The ERK5 protein, which is encoded by the MAPK7 gene, comprises an N-terminal kinase domain and a large C-terminal domain containing transcriptional transactivating functionality and nuclear localization and export sequences (NLS/NES). ERK5 is the effector kinase of a canonical kinase module comprising MEK (MAPK/ERK kinase) 5, MEKK (MEK kinase) 2/3 and ERK5 itself.

The conventional, so-called type I, kinase inhibitor-binding mode is demonstrated by structures of ERK5 co-crystallized with the aminopyrimidine-containing compounds 2 and 3, while a novel allosteric binding mode was observed for three triazole-containing compounds (compounds 4–6). Compounds 2 and 3, like compound 1, bind at the conventional ATP-binding site, while compounds 4, 5 and 6 bind at a novel allosteric binding site. The aminopyrimidine motif forms a hydrogen-bond network with the backbone of Met140 in the ERK5 hinge region. The amide substituent on the phenyl ring of compound 3 extends into the solvent-accessible channel (the so-called front pocket; FP) and the amide NH donates a hydrogen bond to the side-chain amide carbonyl O atom of Gln146. The terminal piperidine ring provides an additional ionic interaction with the likely deprotonated carboxylic acid of Asp143. The N-isopropyl group of compound 3 is positioned similarly to the benzene ring in the 6,7,6 ring systems of compounds 1 and 2. As observed for the complex of compound 1 with ERK5, compounds 2–5 bind to a ‘DFG-in’ conformation of ERK5 in which both the hydrophobic R-spine (residues Leu106, Ile117, His180 and Phe201 in ERK5) and C-spine (Val69, Ala82, Leu144, Leu188, Leu189, Val190, Ile251 and Met255) are intact. The most potent allosteric inhibitor, compound 5, has an IC50 of 2.3 µM in an assay of ERK5 kinase activity, compared with an IC50 of 42 nM for the conventional kinase inhibitor 3. Compounds 2, 3 and 5 were tested against a panel of 225 kinases representative of the kinome to assess the selectivity of these three different scaffolds. The kinase selectivity-profile data show that compound 5 is the most selective, while compound 3 is the most promiscuous, with the selectivity of compound 2 being intermediate.

> TFDVGDEYEIIETIGNGAYGVVSSARRRLTGQQVAIKKIPNAFDVVTNAKRTLRELKILKHFKHDNIIAIKDILRPTVPYGEFKSVYVVLDLMESDLHQIIHSSQPLTLEHVRYFLYQLLRGLKYMHSAQVIHRDLKPSNLLVNENCELKIGDFGMARGLCTSPAEHQYFMTEYVATRWYRAPELMLSLHEYTQAIDLWSVGCIFGEMLARRQLFPGKNYVHQLQLIMMVLGTPSPAVIQAVGAERVRAYIQSLPPRQPVPWETVYPGADRQALSLLGRMLRFEPSARISAAAALRHPFLAKYHDPDDEPDCAPPFDFAFDREALTRERIKEAIVAEIEDFHARREGI> CCTCTGGTCTCC;> 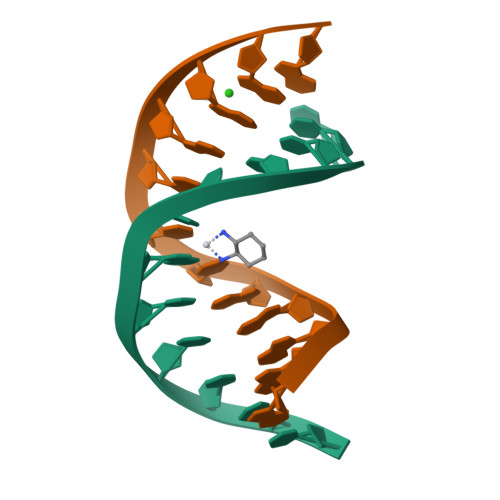GGAGACCAGAGG TrmD (tRNA-(N(1)G37) methyltransferase) is an essential tRNA modification enzyme in bacteria that prevents +1 errors in the reading frame during protein translation and represents an attractive potential target for the development of new antibiotics. TrmD belongs to a distinct class of S-adenosyl-l-methionine (SAM)-dependent methyltransferases known as the SpoU-TrmD (SPOUT) RNA methyltransferase superfamily or Class IV methyltransferases. Each non-crystallographic 2-fold symmetry-related protomer of TrmD interacts in an antiparallel manner and consists of two domains: a larger N-terminal domain spanning residues 1–161 and a smaller C-terminal helical domain (177–242) connected by a flexible inter-domain linker. The SAM binding region of TrmD is located at the base of the N-terminal domain and consists of a deep trefoil knot architecture, made of three distinct untwisted loop regions.

The 4-methoxyphenyl and indole ring systems of Fragments 23 and 24 overlap perfectly, while the 6-boronic acid group of fragment 24 partially extends into the SAM adenine pocket and makes hydrogen bonds with the backbone amides of residues Tyr136 and Leu138 and further water-mediated hydrogen bond contacts to the backbone amides of Val131, Ile133, Gly134 and the side chain hydroxyl group of Ser132. Compound AW1 (Kd 0.11 mM, LE 0.36, IC50 0.23 mM), formed by merging the two fragments, adopts a similar conformation to that of the original fragments in the TrmD SAM site, as shown in Figures 3B, C and Supplementary Figure S4, thereby providing a new chemical scaffold for further structure-guided development. While the observed fragment hits and the corresponding merged compound AW1 satisfy many of the predicted protein-hotspot interactions, the map also suggested further potential interactions that could stabilise elaborated fragments. AW1 occupies Hotspot 1 at the base of the TrmD active site, where it satisfies the hydrogen-bond donor requirements by interacting with the backbone amide oxygen atoms of Gly134 and Tyr136. The merged compound AW1 also orients its pyrazole nitrogen atom in the acceptor map in this region where it forms a hydrogen bond with the backbone NH of Leu138. The compound could be elaborated further towards the methionine end of the active site and by further extension to the second hotspot region at the top of the active site. Structure-guided elaboration of the merged compound AW1 (Kd 0.11 mM, LE 0.36, IC50 0.23 mM) was performed, initially utilizing the indole nitrogen as a vector for growth.

>GSMKIDVVTIFPEYLQPVRQSLPGKAIDAGLVDVAVHDLRRWTHDVHKSVDDSPYGGGPGMVMKPTVWGDALDEICTSETLLVVPTPAGYPFTQETAWQWSTEDHLVIACGRYEGIDQRVADDAATRMRVREVSIGDYVLNGGEAAALVIIEAVLRLVPGVLGNALSAQEDSHSEGMASLLEGPSYTRPPSWRGMDVPPVLLSGDHAKIAAWRAEQSRQRTIERRPDLLGFDSPTGEHGGDGLS[2x]1,3-dimethoxy-8-oxidanyl-anthracene-9,10-dione | C16 H12 O5 | 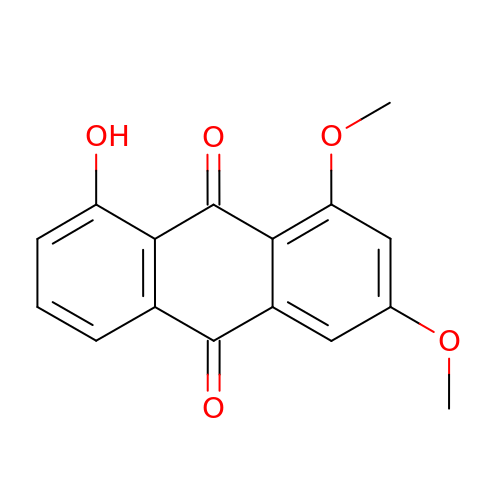MCHNUYTWURIGNT-UHFFFAOYSA-N> MLDLKISQSKIALPKNTVGGTILRSDLLANFLTEGNFRASVDLQRTHRIKGMIKMVATVGIPENTGIALACAMNSSIRGRASSDIYTICSQ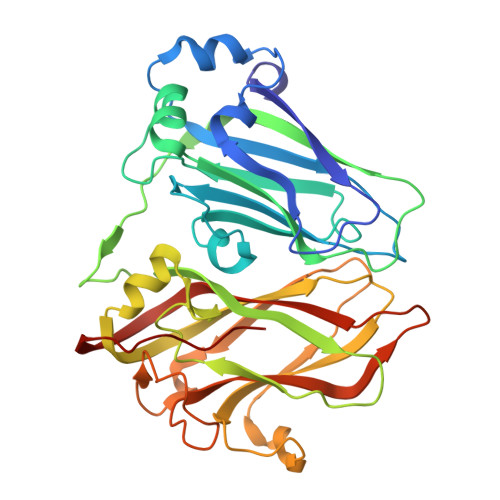DCELWNPACTKAMTMSFNPNPCSDAWSLEFLKRTGFHCDIICVTGWTATPMQDVQVTIDWFISSQECVPRTYCVLNPQNPFVLNRWMGKLTFPQGTSRSVKRMPLSIGGGAGAKSAILMNMPNAVLSMWRYFVGDLVFEVSKMTSPYIKCTVSFFIAFGNLADDTINFEAFPHKLVQFGEIQEKVVLKFSQEEFLTAWSTQVRPATTLLADGCPYLYAMVHDSSVSTIPGDFVIGVKLTIIENMCAYGLNPGISGSRLLG> MIRGSSALKSLTSRRLYSTGVKYTTLSNGVTVATETNPAAKTSSVGLFFGAGSRSEHSHSNGISALTTNVLASQSAKGSLLTAKNDREFNGIIAQTTNDNITEAGKLIASIASNAVDIVEKTDLTKHKQYLSAQASAVEADPKSKVLSHLYSSAFQGYSLALPTLGTTESVENLENQDSLRHLAKHLVNNNTVIAASGNFDHDKLADAIEANLKIAEGVKPEIKPASFLGSEVRMRDDTLPKAYISIAVHGEGLNSPNYYLAKVAAAIYGDFYLHSTIAKFTSPKLASIVQEYNIVESYNHYSKSFSDTGIWGYYAEIADKFTVDDFTHFSLKEWNRLSISISEAEVARAKAQVKTALAKELANSFAVTSDIAEKVLLVGHRQSLREAFEKIDAIKVNDVKEWGKSKVWDRDIVISGTGLIEDLLDYNRNRNEMAMMRW;> MLSRASIRAYSSIPNSVKIAAKESATDLTKLSVIINNAGSKTGKSGVSHLLSKFTFLNNGAKSALRFTRESELLGGTFESKVTRDALILNTTFLKQDLPYYVEALGNVVSNTQFAPHEFNEIVLPTANAETKLANANPAFKGVEKLHEITFRRGLGNPLFYNESTPIKLEEVAQFSKEQFSGENISIVAEGANEEDLTKFVSESAFCYLPSSSSNGAKALPTNTFTGQEARVPSSGASSALIGIPVKPADFGKYEVLSAAIGTSTLPSTSTPLAQIPGATSHLYKYQDAGLFVISVSGEASQVAQGIKQAKSVAESVSSSALSEAVKAAELSVALQSTVDSPLNVKVVAEEAPISKFNYVAVGDLDVLPYADEL;> MFRTAYKTMNQSMVQKFIAGGVGVTGLTASYLLYQDSMTADAMTAAEHGLHPPAYNWPHNGMFETFDHASIRRGFQVYREVCAACHSLDRIAWRNLVGVSHTTSEAKAMAEELEYDDEPDDEGKPRKRPGKLADYIPGPYENEQAARAANQGAYPPDLSLIVKARHGGSDYIFSLLTGYPDEPPAGVVLPEGSNYNPYFPGGAIAMGRVLFDDLVEYEDGTPATTSQMAKDVSTFLNWASEPEHDDRKKWGLKALVVLSSLYLLSIWVKRFKWTPIKNRKFRFDPPKK;>[2x]MSSLAFRTLRNGLGLKSSVRALSTTTTTLSNYQQPDYSSYLNNKSGQGSRNFTYFMVGSMGLLSAAGAKSTVEAFLSSFAASADVLAMAKVEVKLGAIPEGKNVIIKWQGKPVFIRHRTADEIEEANQVDIKTLRDPQNDADRVKKPEWLIMLGICTHLGCVPIGEAGDFGGWFCPCHGSHYDISGRIRKGPAPLNLEIPEYDFTDDETLLVG;> MAGAPHPHTYMGWWGSLGSPKQKYITQYTISPYAAKPLKGAAYNAVFNTFRRTKNQFLYVAIPFVVVWSIWTRARDYNEYLYTKEGREELERVNV;> MVQSMTSVVKAANFILARPTLSKIITPLAQKFTAYAGYREMGLKFNDLLLEETPIMQTAIKRLPSELNYSRNFRILTAHQLALSHQLLPAEKAVKPEEDDNYLIPYILEAEKEAFEKAELDNIEVKA;> MSFFRDLLESVVPTAYAEEPVEDVEVEQPEDAPEEEVSEETVEEEEEDDEDDDEDDEEEEETADPLDTLREECTKTAACKPFDHHFHECIERVTKEQEEPDYEHKHYKEDCIEEFFHLQHCVNDCVAPRLFNRLK;> MLTVLGRLLERNSIYVATIFGGAFAFQGFFDVAVNKWWEEHNKAKLWKNVKGKFLEGEGEEEDDE;> MPTRKSNTYLSLVNSYLIDSPQPSSINYWWNLGSLLGLCLVIQIASGVFLAMHYSSNIELAFDSVEHIMRDVNAGWLIRYIHANGASFFFICMYLHIGKALYYGSYKQPRVMLWVIGVVIFILTMAIAFMGYCLVYGQMSHWGATVITNLLSAIPFIGNDIVPFIWGGFSVSNPTIQRFFALHFLLPFILAALVCMHLM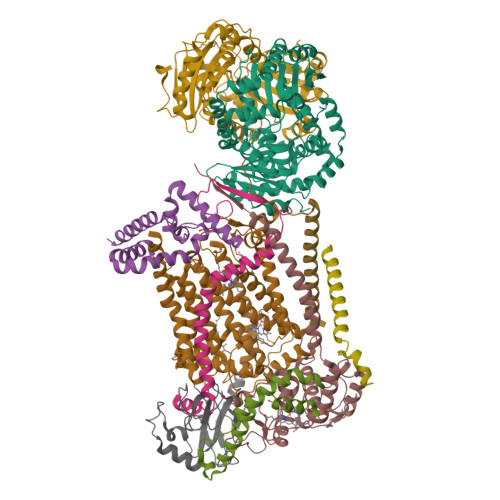ALHVHGSSNPVGITGNIDRLPMHPYFIFKDLITVFVFLLIFSLFVFYSPNTLGHPDNYIPGNPMVTPPSIVPEWYLLPFYAILRSIPDKLGGVIAMFGAILILLSLPYTDRSIIRGNSFKVLSKLAFYLFVFNFILLGNLGQLHVEVPYIQLGQFATAYYFAHYIIVVPVISTLENILYYIGTQTRVK>MATAHFVLIHTI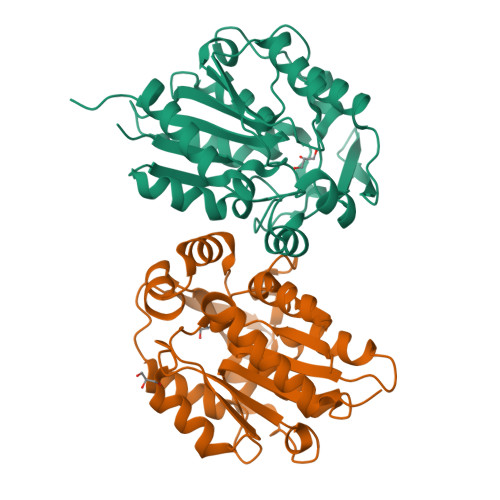CHGAWIWYKLKPLLEAAGHKVTALDLAASGIDPRQIEQINTFDEYSEPLLTFMESLPQGEKVILVGESCGGLNIALAADKYPEKISAAVFHNALMPDTEHSPSYVVDKFMEVFPDWKDTEFSTYTSNNETITGMKLGFKLMRENLYTNCPIEDYELAKMLTRKGSFFQNDLAQRPKFTEEGYGSIKRVYVWTDEDKIFPPEFQLWQIENYKPDKVYRVQGGDHKLQLSKTNELAEILQEVADTYADLLAVAGLEHHHHHH[4x]> METNLFKLSLDDVETPKGSMLDLKISQSKIALPKNTVGGTILRSDLLANFLTEGNFRASVDLQRTHRIKGMIKMVATVGIPENTGIALACAMNSSIRGRASSDIYTICSQDCELWNPACTKAMTMSFNPNPCSDAWSLEFLKRTGFHCDIICVTGWTATPMQDVQVTIDWFISSQECVPRTYCVLNPQNPFVLNRWMGKLTFPQGTSRSVKRMPLSIGGGAGAKSAILMNMPNAVLSMWRYFVGDLVFEVSKMTSPYIKCTVSFFIAFGNLADDTINFEAFPHKLVQFGE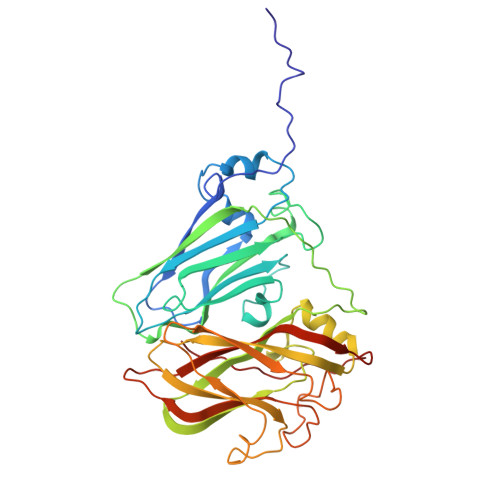IQEKVVLKFSQEEFLTAWSTQVRPATTLLADGCPYLYAMVHDSSVSTIPGDFVIGVKLTIIENMCAYGLNPGISGSRLLGTIPQ> MSPKLPQHGTVGVRTPLVDGVEKVTGKAKYTADIAAPDALVGRILRSPHAHARILAIDTSAAEALEGVIAVCTGAETPVPFGVLPIAENEYPLARDKVRYRGDPVAAVAAIDEVTAEKALALIKVDYEVLPAYMTPKAAMKAGAIALHDDKPNNILREVHAEFGDVAAAFAEADLIREKTYTFAEVNHVHMELNATLAEYDPVRDMLTLNTTTQVPYYVHLKVAACLQMDSARIRVIKPFLGGGFGARTEALHFEIIAGLLARKAKGTVRLLQTREETFIAHRGRPWTEVKMKIGLKKDGKIAALALEATQAGGAYAGYGIITILYTGALMHGLYHIPAIKHDAWRVYTNTPPCGAMRGHGTVDTRAAFEALLTEMGEELGIDSLKIRQINMLPQIPYVTMYAQRVMSYGVPECLEKVKAASGWEERKGKLPKGRGLGIALSHFVSGTSTPKHWTGEPHATVNLKLDFDGGITLLTGAADIGQGS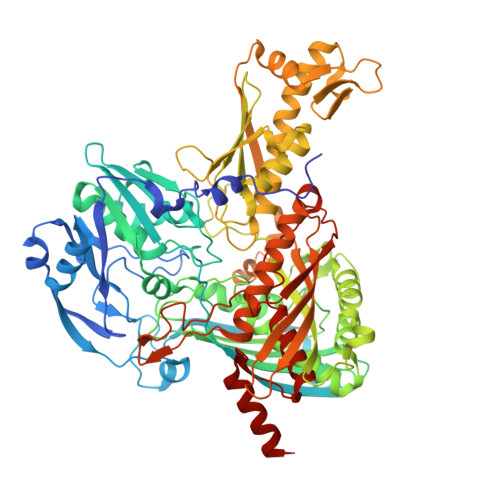NTMASQVAAEVLGVRLSRIRVISADSALTPKDNGSYSSRVTFMVGNASISAAEELKGVLVKAAAKKLDAREEDIEVIDEMFMVSGSQDPGLSFQEVVKAAMVDSGTITVKGTYTCPTEFQGDKKIRGSAIGATMGFCYAAQVVEASVDEITGKVTAHKVWVAVDVGKALNPLAVEGQTQGGVWMGMGQALSEETVYDNGRMVHGNILDYRVPTIVESPDIEVIIVESMDPNGPFGAKEASEGMLAGFLPAIHEAVYEAVGVRATDFPLSPDRITELLDAKEAAA> MPLDSILVDNVALQFF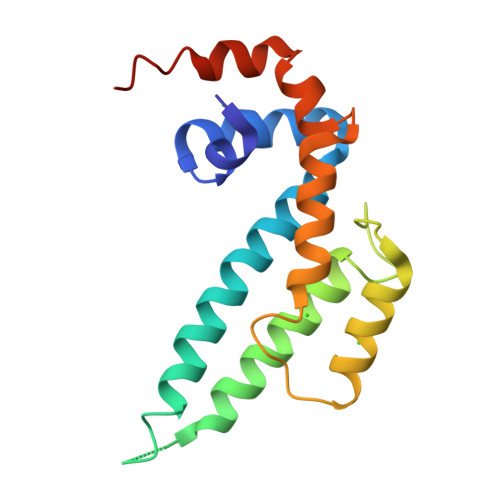MDYMQQTGGQAHLFFWMTVEGYRVTAQQQLEVLLSRQRDGKHQTNQTKGLLRAAAVGIYEQYLSEKASPRVTVDDYLVAKLADTLNHEDPTPEIFDDIQRKVYELMLRDERFYPSFRQNALYVRMLAELEHHHHHH> GPAMHEFVSGTPGKELPQEVKDLLPADQTDLKDGSQSTPTQPSKTEVKTAEGTWSFKSYDKTSETINEADVHFVGTWEFTPAPTYKAT

Here, we show that repeat number variation in predicted bacterial surface proteins is more widespread and we characterize a third rod-like repetitive region in the Streptococcus gordonii protein (Sgo_0707) formed by tandem array of Streptococcal High Identity Repeats in Tandem (SHIRT) domains. The structure of single and tandem SHIRT domains from the streptococcal surface protein Sgo_0707 were determined. We call SasG, Rib, and Sgo_0707 “Periscope Proteins” due to their having variable-length stalk-like regions that define the distance that the N-terminal functional domain projects from the bacterial surface. Taken together, these data are consistent with multiple tandemly arrayed SHIRT domains from Sgo_0707 behaving as an elongated, rod-like particle.

Defining the structural, rather than sequence, repeat boundaries in repetitive bacterial proteins is challenging. For Sgo_0707 the T-REKS server predicts a repeat frame of 460 through 543 and 13 repeats of 84 through 90 residues. A construct based on the second repeat (residues 544 through 627; ΔN-Sgo_R2) was folded and solved to 0.95 Å resolution using X-ray crystallography utilizing ab initio molecular replacement (MR) with ideal fragments. Based on the significant truncation of the N-terminal β-strand (Inset), we hypothesized that shifting the frame of the repeat by seven residues toward the N terminus of Sgo_0707 would complete the fold.>MGSDKIHHHHHHENLYFQGMVKHIVLFKLRDDVPVEEKLVVMNSFKEAIEALPAKISVIRKIEVGLNMNPGETWNI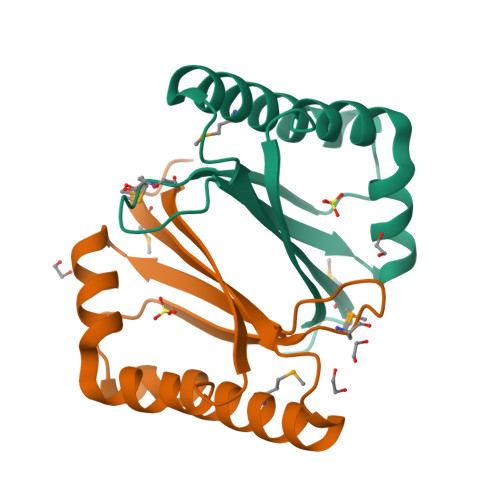ALYSEFDNLDDVKFYATHPEHVAAGKILAETKESRACVDYEF[2x]> YVEIIEQPKQRGMRFRYKCEGRSAGSIPGERSTDTTKTHPTIKINGYTGPGTVRISLVTKDPPHRPHPHELVGKDCRDGFYEA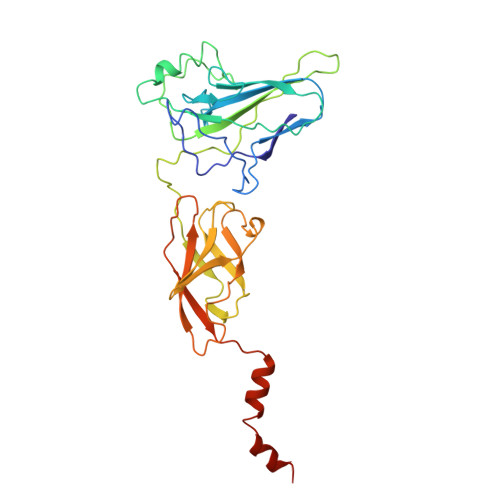ELCPDRCIHSFQNLGIQCVKKRDLEQAISQRIQTNNNPFQVPIEEQRGDYDLNAVRLCFQVTVRDPSGRPLRLPPVLPHPIFDNRAPNTAELKICRVNRNSGSCLGGDEIFLLCDKVQKEDIEVYFTGPGWEARGSFSQADVHRQVAIVFRTPPYADPSLQAPVRVSMQLRRPSDRELSEPMEFQYLPDTDDRHRIEEKRKRTYETFKSIMKKSPFSG> GGGUUGUAUAAGCUCGUUAAUUUGGAAUGAGCGUAUCUACAGGCAACCGUAAAUUGCCCCAGGCUACAA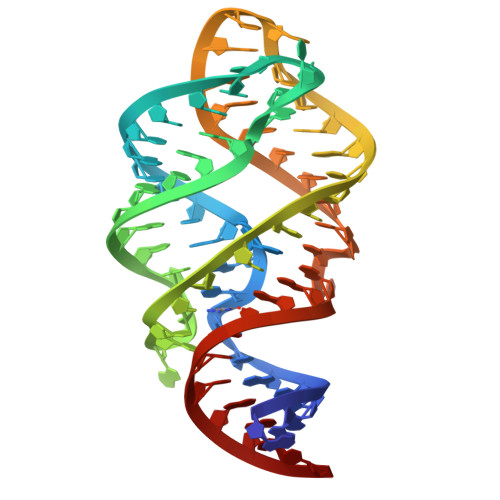UC>[60x]GGGGIGVSTGTYDNQTTYKFLGDGWVEITAHASRLLHLGMPPSENYCRVTVHNNQTTGHGTKVKGNMAYDDTHQQIWTPWSLVDANAWGVWFQPSDWQFIQNSMESLNLDSLSQELFNVVVKTVTEQQGAGQDAIKVYNNDLTACMMVALDSNNILPYTPAAQTSETLGFYPWKPTAPAPYRYYFFMPRQLSVTSSNSAEGTQITDTIGEPQALNSQFFTIENTLPITLLRTGDEFTTGTYIFNTDPLKLTHTWQTNRHLGMPPRITDLPTSDTATASLTANGDRFGSTQTQNVNYVTEALRTRPAQIGFMQPHDNFEANRGGPFKVPVVPLDITAGEDHDANGAIRFNYGKQHGEDWAKQGAAPERYTWDAIDSAAGRDTARCFVQSAPISIPPNQNQILQREDAIAGRTNMHYTNVFNSYGPLSAFPHPDPIYPNGQIWDKELDLEHKPRLHVTAPFVCKNNPPGQLFVRLGPNLTDQFDPNSTTVSRIVTYST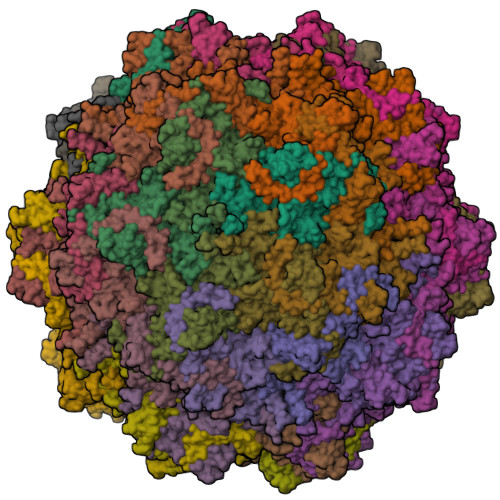FYWKGILKFKAKLRPNLTWNPVYQATTDSVANSYMNVKKWLPSATGNMHSDPLICRPVPHMTY>[2x]STLSDGIYTIPFVAKKANDDS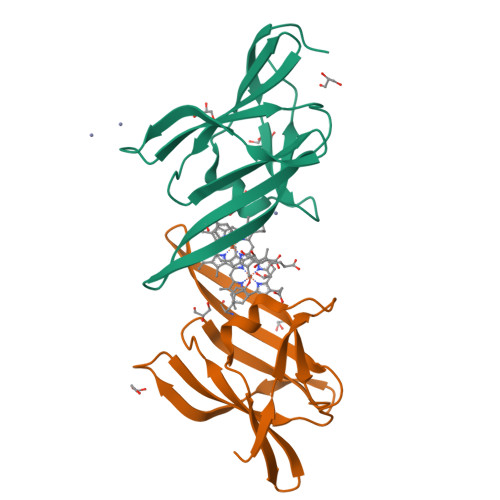NSSMQNYFNNPAWLKVKNGKKMVAMTVNDNKTVTALKTTLAGTLQDVKVVSEDKDANTRIVEFEVEDLNQPLAAHVNYEAPFNGSVYKGQADFRYVFDTAK> MPVRRGHVAPQNTFLDTIIRKFEGQSRKFIIANARVENCAVIYCNDGFCELCGYSRAEVMQRPCTCDFLHGPRTQRRAAAQIAQALLGAEERKVEIAFYRKDGSCFLCLVDVVPVKNEDGAVIMFILNFEVVMEKDMVGSGADVLPEYKLQAPRIHRWTILHYSPFKAVWDWLILLLVIYTAVFTPYSAAFLLKETEEGPPATECGYACQPLAVVDLIVDIMFIVDILINFRTTYVNANEEVVSHPGRIAVHYFKGWFLIDMVAAIPFDLLIFGSGSEELIGLLKTARLLRLVRVARKLDRYSEYGAAVLFLLMCTFALIAHWLACIWYAIG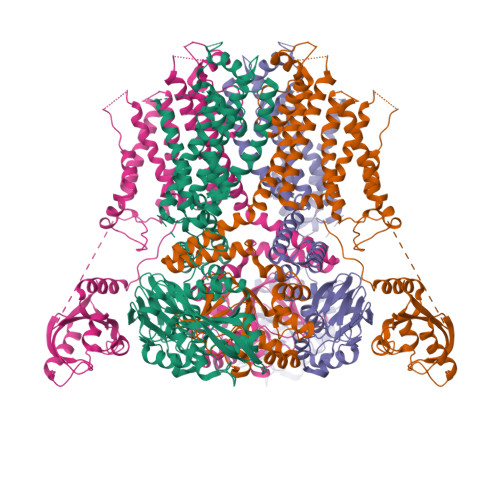NMEQPHMDSRIGWLHNLGDQIGKPYNSSGLGGPSIKDKYVTALYFTFSSLTSVGFGNVSPNTNSEKIFSICVMLIGSLMYASIFGNVSAIIQRLYSGTARYHTQMLRVREFIRFHQIPNPLRQRLEEYFQHAWSYTNGIDMNAVLKGFPECLQADICLHLNRSLLQHCKPFRGATKGCLRALAMKFKTTHAPPGDTLVHAGDLLTALYFISRGSIEILRGDVVVAILGKNDIFGEPLNLYARPGKSNGDVRALTYCDLHKIHRDDLLEVLDMYPEFSDHFWSSLEITFNLRDTNMIPGGRQYQELPRCPAPTPSLLNIPLSSPGRRPRGDVESRLDALQRQLNRLETRLSADMATVLQLLQRQMTLVPPAYSAVTTPGPGPTSTSPLLPVSPLPTLTLDSLSQVSQFMACEELPPGAPELPQEGPTRRLSLPGQLGALTSQPLHRHGSDPGSEASNSLEVLFQ7-NITROINDAZOLE-2-CARBOXAMIDINE | C8 H7 N5 O2 | 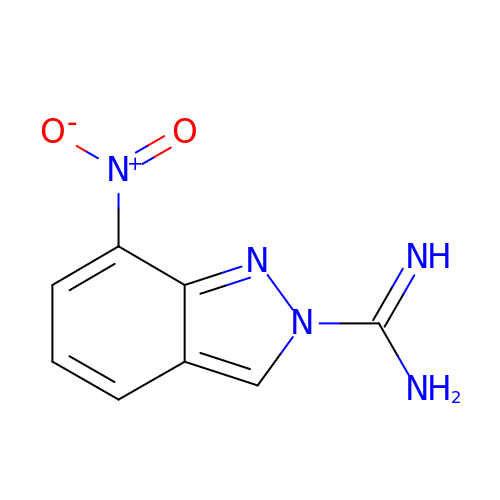GFYAZUABYOOPCN-UHFFFAOYSA-N>GSHMAVQIGFLLFPEVQQLDLTGPHDVLASLPDVQVHLIWKEPGPVVASSGLVLQATTSFADCPPLDVICIPGGTGVGALMEDPQALAFIRQQAARARYVTSVCTGSLVLGAAGLLQGKRATTHWAYHELLAPLGAIPVHERVVRDGNLLTGAGITAG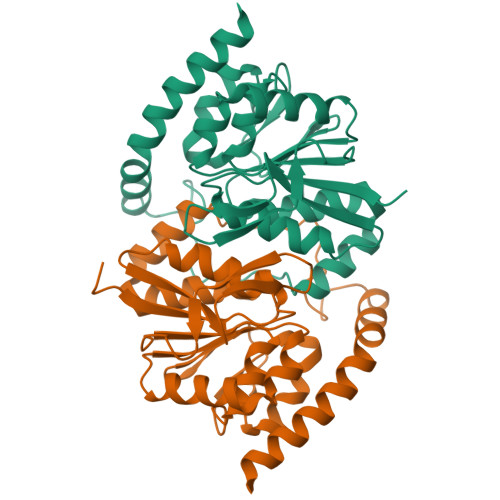IDFALTLAAELFDAATAQRVQLQLEYAPAPPFNAGSPDTAPASVVQQARQRAADSLHKRREITLRAAARLAAG[2x]> MRRLSVSFLPFHLIVTTQRRQFGGNSKDGHKGEDKPIERVGEVPPTGPHPFNITSGAEGQISNQQRKAHDAITQLFRDDAQRKALYQKPGRTIGAQTTTAAISTPPNEDEFEGLQPISGDAE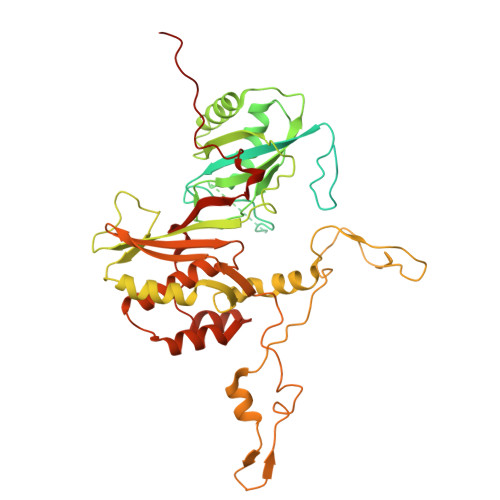PSSITAVEAVEQELLDDAFLYFPPAQQSASGSVATTATNELYVPGQQIIPPGLTRYRVDVQYQGNDFDGWWKSTTRQLFRREVGLDGSITRVPVAEPGTIGNAAGASRGETMGSRYHARTVLEEALAVALDVNTVRVVAGVIPEVGVSVRRLCCHVDVPSHIELQPRTVIQRATMWMEKRQQPLAILSYRRCKNQDFHARHSGLRRVYVYRILNRVAPPLFDAGLQWHVDRHLDVDRMKRFAKALEGTKDFGYFADPKMANALRRAAMSPGGFSTGAVTEENFQPKATGESHRVTRGKAPKVTMEKGPSNLDRAAALPTFNEYGQRVVQPGAHGKEYYRVATNLPTVRTVDRLDVVRQDDEVLIWFVGRSFLRHQIRNMVSVLKAAGHGLWNDLELQQALQSGFEPSRHRFKRERFPTAPAYGLTLWDVEYPDQHRDDYVQFVDSGPYEQVNIARDI> MASNIESALANRTMGRGRAPGKTIAVNYQAAS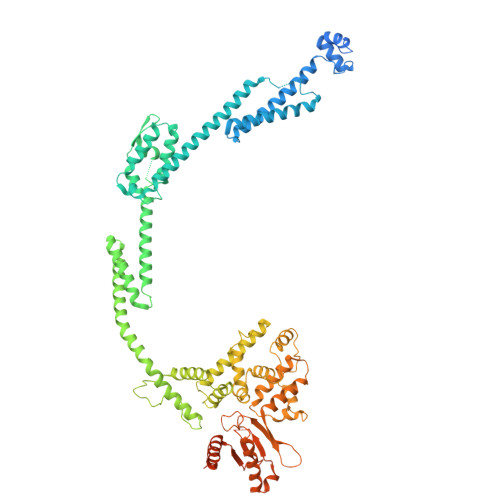VQAPTGDSGLARALTSFVESGTGLYKQFKDEEKTRADERSNEIIRKLTPQQRREAIQNGTLLYQDDPYAMEALRVKTGRNAAFAVDDEINVKIQNGEFRTRQDMEEYRHQRLQDAAKSYAEEAGINPTDEFFQRGFNDNITDRNIAIYGSFNKYFSKQSEETAMLNTRIEMNSFLNDGDLMRSPESGKTFMAYLRDGLTTAAIPSDQRAREVITQTVRDAIQKSGGSNFLQQVRGERITLNGVDATVEEIVGPDVFNAAIVEAQGTEYKLVAKYQEDLALGVQSAILQDDPTIGLAQIQKLKEQNNLLQPGEELTPQRQMLINAEASLLEAVKRKSAEQAKENTKLIQTQNKQLVIDQVYQRRLAGDNVSTNYEDLPVSEATGEFKRSDMNNYASAKLQQIDQMDIPEAAKDAQKVALLRADTNNGPFRNAFQTLTQDAAGEWQAAVIRGQYDPDKMQRFESLRRAYTQDPSSFAALYPDQAQLFSTFDQMDKIGLDPQTMIEADKQAASQSREMRMESDKAWQELKNDSRNKDLSRLPTSLDASARKVWDSWYYRTGNADAATQQTQRWLNENTVTFQSEGSDGKSIGMVSKHQLMVGDNPESWQVGRDIIDTARKQLIKANPWVVNSQLSVVEQNGSIFLQDATGTIRIRYDKELVGKLYREQQQKAQDAAYAQAERDANKRARIVGTKAAGDKRRADREANIEKRGGMYNDVSLEGIAKVLIGKE> LEADKCKEREEKIILVSSANEIDVRPCPLNPNEHKGTITWYKDDSKTPVSTEQASRIHQHKEKLWFVPAKVEDSGHYYCVVRNSSYCLRIKISAKFVENEPNLCYNAQAIFKQKLPVAGDGGLVCPYMEFFKNENNELPKLQWYKDCKPLLLDNIHFSGVKDRLIVMNVAEKHRGNYTCHASYTYLGKQYPITRVIEF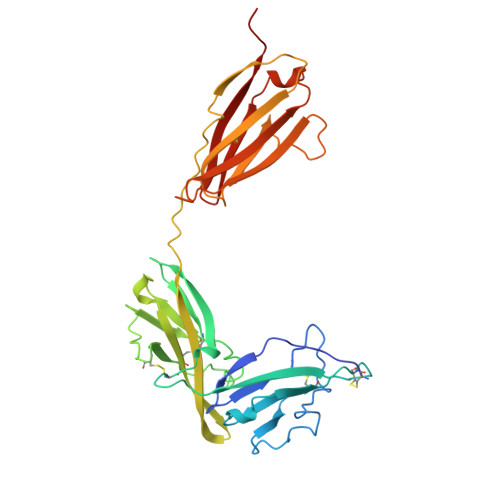ITLEENKPTRPVIVSPANETMEVDLGSQIQLICNVTGQLSDIAYWKWNGSVIDEDDPVLGEDYYSVENPANKRRSTLITVLNISEIESRFYKHPFTCFAKNTHGIDAAYIQLIYPVT> MTNIEPVIIETRLELIGRYLDHLKKFENISLDDYLSSFEQQLITERLLQLITQAAIDINDHILSKLKSGKSYTNFEAFIELGKYQILTPELAKQIAPSSGLRNRLVAEFDDIDPNQVFMAISFALQQYPLYVRQINSYLITLEEENDLESGHHHHHH;> MQDKIPTIAELRELSLRLLTKIPYLKMLVLFGSRAT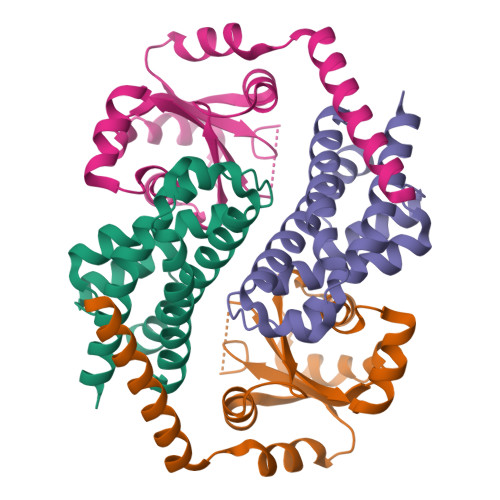GNINANSDWDFAVLYDEEKYNLYIQNNPLAAFVIPGILGEIFKINSDKIDIVELNHCSKLIAHFVARDGKVLYEEPGDEFDKFQQRVLLSNTEIKKIEKTKLENIENFLQRWGV>[2x]HHHHHHFNLPPGNYKKPKLLYCSNGGHFLRILPDGTVDGTRDRSDQHIQFQLSAESVGEVYIKSTETGQYLAMDTDGLVYGSQTPNEE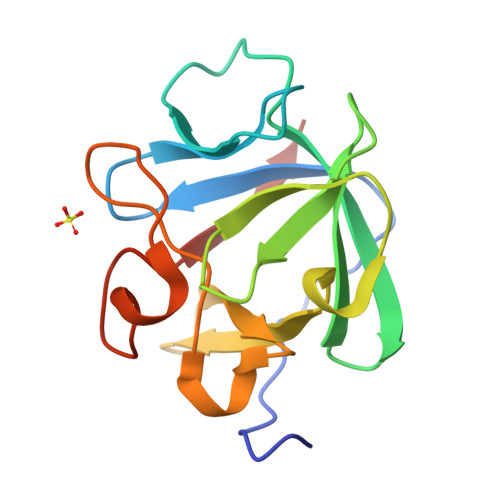CLFLERLEENHYNTYISKKHAEKNWFLGLKKNGSVKRGPRTHYGQKAILFLPLPVSSD The toxin of the system (DarT) is a domain of unknown function (DUF) 4433, and the antitoxin (DarG) a macrodomain protein. We demonstrate that DarT is an enzyme that specifically modifies thymidines on single-stranded DNA in a sequence-specific manner by a nucleotide-type modification called ADP-ribosylation. We also show that this modification can be removed by DarG. The DarG macrodomain adopts a typical macrodomain fold composed of a six-stranded mixed β sheet sandwiched between four α helices and one 310-helical element.

To get a better understanding of the antitoxin function, we determined the high-resolution X-ray crystal structures of the Taq and Mtb DarG macrodomains (TaqDarG-macro and MtbDarG-macro) in a ligand-free or ADPr-bound form. TaqDarG-macro and MtbDarG-macro share the same overall structure with an RMSD (root-mean-square deviation) of 0.89 Å over 149 α-carbons and a 56.4% sequence identity. To probe the requirements for the de-ADP-ribosylation activity of DarG, we devised constructs with substitutions of conserved and ADPr pocket-facing amino acids. While some of the mutations (H82A and W83A) showed little or no effect on the de-ADP-ribosylation activity of TaqDarG after 21 min, others (N22A, K29E, G119E, and K80A) had marked inhibitory effects. Interestingly, mutation of K80, the equivalent of the main catalytic lysine residue in TARG1, showed the most significant effect on substrate turnover out of all the mutants tested and resulted in inactive TaqDarG, indicating that this feature is conserved between TARG1 and DarG (Sharifi et al., 2013). N22A showed the most significant effect on substrate turnover after K80A, and because of its location and the effect of its mutation on the enzyme’s activity, it might be involved in the positioning and binding of the ADP-ribosylated thymidine moiety. The reduced catalytic activity observed in the G119E mutant is most likely due to the position of the residue in one of the loops involved in ligand binding. This loop undergoes a conformational change between residues 117 to 122 in order to grasp the ADPr moiety upon ligand binding, with a maximum distance variation of 7.66 Å between the α-carbon of Gly121 in both states.

> MGHHHHHHGGMLRFVRGNLLEAPVEALVNTVNTVGVMGKGVALQFKRAFPDNYQAYVKACERGQVQIGRIFVYDRGPLAQPRYIFNFPTKKHWRHPSRMEYVEEGLKDLVCRIQELRVRSIALPPLGAGNGGLPWPEVKQRIQEALEALEGVEVWVYEPVENPKA N-({3-HYDROXY-2-METHYL-5-[(PHOSPHONOOXY)METHYL]PYRIDIN-4-YL}METHYL)-2-METHYL-L-GLUTAMIC 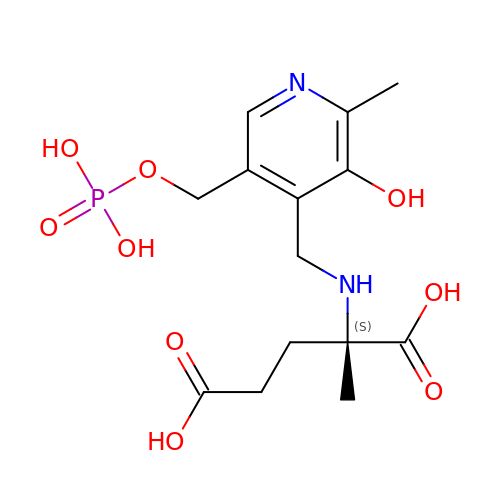ACID | C14 H21 N2 O9 P | CNIVMJHNGQZEAY-AWEZNQCLSA-N>MVSKNKKLNLKDKYQYLTRDMAWEPTYQDKKDIFPEEDFEGIKITDWSQWEDPFRLTMDAYWKYQAEKEKKLYAIFDAFAQNNGHQNISDARYVNALKLFISGISPLEHAAFQGYSKVGRQFSGAGARVACQMQAIDELRHSQTQQHAMSHYNKHFNGLHDGPHMHDRVWYLSVPKSFFDDARSAGPFEFLTAISFSFEYVLTNLLFVPFMSGAAYNGDMATVTFGFSAQSDEARHMTLGLEVIKFILEQHEDNVPIVQRWIDKWFWRGFRLLSLVSMMMDYMLPNKVMSWSEAWEVYYEQNGGALFKDLERYGIRPPKYQDVANDAKHHLSHQLWTTFYQYCQATNFHTWIPEKEEMDWMSEKYPDTFDKYYRPRYEYLAKEAAAGRRFYNNTLPQLCQVCQIPTIFTEKDAPTMLSHRQIEHEGERYHFCSDGCCDIFKH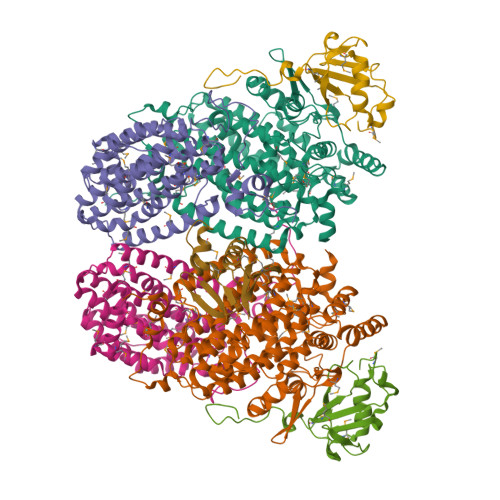EPEKYIQAWLPVHQIYQGNCEGGDLETVVQKYYHINIGEDNFDYVGSPDQKHWLSIKGRKPADKNQDDA[2x];>[2x]MSIEIKTNSVEPIRHTYGHIARRFGDKPATRYQEASYDIEAKTNFHYRPQWDSEHTLNDPTRTAIRMEDWCAVSDPRQFYYGAYVGNRAKMQESAETSFGFCEKRNLLTRLSEETQKQLLRLLVPLRHVELGANMNNAKIAGDATATTVSQMHIYTGMDRLGIGQYLSRIALMIDGSTGAALDESKAYWMDDEMWQPMRKLVEDTLVVDDWFELTLVQNILIDGMMYPLVYDKMDQWFESQGAEDVSMLTEFMRDWYKESLRWTNAMMKAVAGESETNRELLQKWIDHWEPQAYEALKPLAEASVGIDGLNEARAELSARLKKFELQSRGVSA;>MSVNALYDYKFEPKDKVENFHGMQLLYVYWPDHLLFCAPFALLVQPGMTFSALVDEILKPATAAHPDSAKADFLNAEWLLNDEPFTPKADASLKEQGIDHKSMLTVTTPGLKGMANAGY[2x];> MSQLVFIVFQDNDDSRYLAEAVMEDNPDAEMQHQPAMIRIQAEKRLVINRETMEEKLGRDWDVQEMLINVISIAGNVDEDDDHFILEWN>[3x]GTKQEKTALNMARWIRSQTLTLLEKLNELDADEQADICES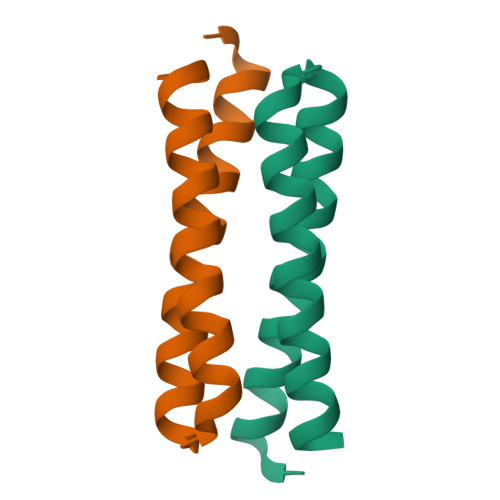LHDHADELYRSCLARFGDDGENL>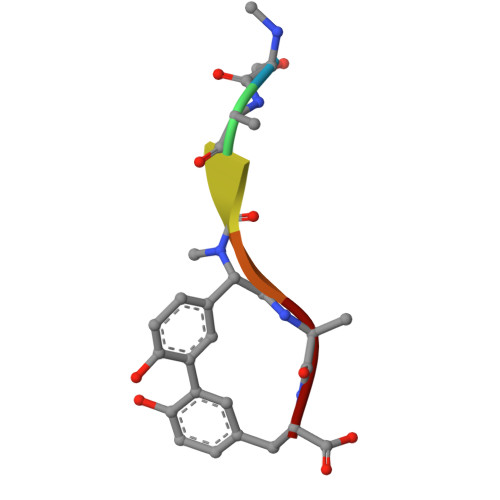 SAGGAY>MVMQNLDRDVVIVGAGPSGLTAARELKKAGLSVAVLEARDRVGGRTWTDTIDGAMLEIGGQWVSPDQTVLMELLDELGLKMYSRYRDGESVYIGADGKRTQYTGDTFPVNETTKAEMDKLVAILDELAAEIGPTEPWAHPKARELDTISFHHWLRQNSNDEEACNNIGLFIAGGMLTKPAHAFSALQAVLMAASAGSFSHLTDEDFILDKRVIGGMQQVSLLQAAELGDDVVLNSPVRTIKWDENGVSVVSERATVNARFVIMAVPPNLYSRVSFDPPLPRRQHQMHQHQSLGLVIKVHAVYDTPFWREEGLSGTGFSAGALVQEVYDNTNHGDSRGTLVGFVSDEKADAVFELSAEDRKKAILESIAGFLGDKALTPEVYYESDWGSEEWTRGAYASSYDLGGLHR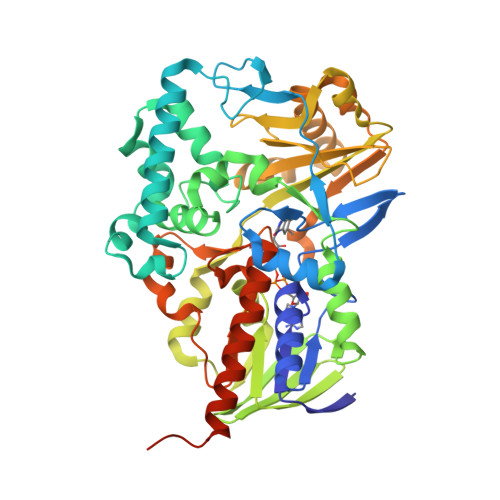YGKDQHANVGPIYWSSSDLAAEGYQHVDGAVRMGQATAARIVEANKLASVPVAAENLYFQSHHHHHHWSHPQFEK[2x]>QGHALKATIYKATVNVADLDRNQFLDASLTLARHPSETQERMMLRLLAWLKYADERLQFTRGLCADDEPEAWLRNDHLGIDLWI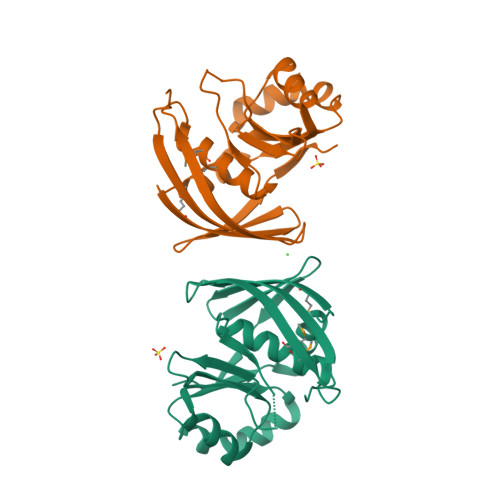ELGLPDERRIKKACTQAAEVALFTYNSRAAQIWWQQNQSKCVQFANLSVWYLDDEQLAKVSAFADRTMTLQATIQDGVIWLSDDKNNLEVNLTAWQQPS[2x]[9-(2-carboxyphenyl)-6-(dimethylamino)xanthen-3-ylidene]-dimethyl-azanium | 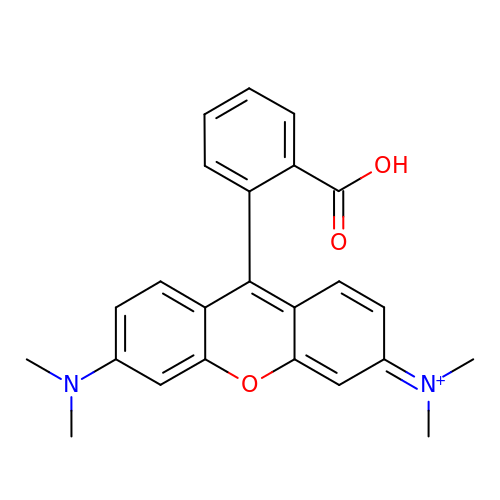C24 H23 N2 O3 | ABZLKHKQJHEPAX-UHFFFAOYSA-O>[2x]MRIIMPVEFSRIVRDVERLIAVEKYSLQGVVDGDKLLVVGFSEGSVNAYLYDGGETVKLNREPINSVLDPHYGVGRVILVRDVSKGAEQHALFKVNTSRPGEEQRLEAVKPMRILSGVDTGEAVVFTGATEDRVALYALDGGGLRELARLPGFGFVSDIRGDLIAGLGFFGGGRVSLFTSNLSSGGLRVFDSGEGSFSSASISPGMKVTAGLE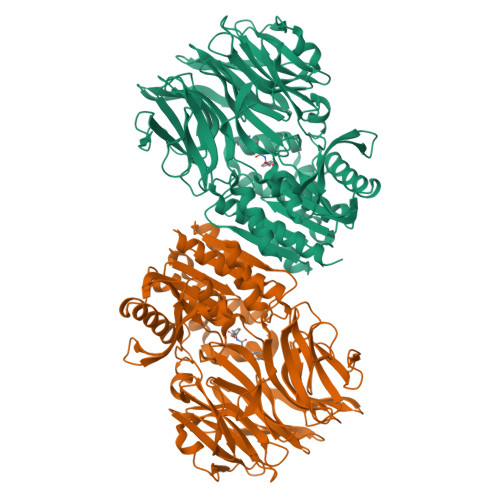TAREARLVTVDPRDGSVEDLELPSKDFSSYRPTAITWLGYLPDGRLAVVARREGRSAVFIDGERVEAPQGNHGRVVLWRGKLVTSHTSLSTPPRIVSLPSGEPLLEGGLPEDLRRSIAGSRLVWVESFDGSRVPTYVLESGRAPTPGPTVVLVHGGPFAEDSDSWDTFAASLAAAGFHVVMPNYRGSTGYGEEWRLKIIGDPCGGELEDVSAAARWARESGLASELYIMGYAYGGYMTLCALTMKPGLFKAGVAGASVVDWEEMYELSDAAFRNFIEQLTGGSREIMRSRSPINHVDRIKEPLALIHPQNDSRTPLKPLLRLMGELLARGKTFEAHIIPDAGHAINTMEDAVKILLPAVFFLATQRERR> DIPQTKQDLELPKLAGTWHSMAMATNEISLMATLKAPLRVHITSLLPTPEDNLEIVLHRWENNSCVEKKVLGEKTENPKKFKIN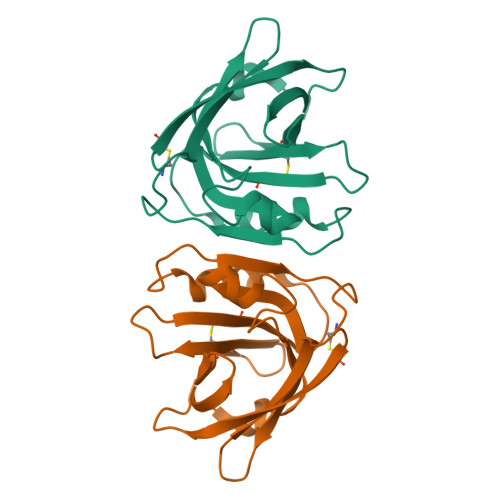YTVANEATLLDTDYDNFLFLCLQDTTTPIQSMMCQYLARVLVEDDEIMQGFIRAFRPLPRHLWYLLDLKQMEEPCRGSAHHHHHH>MYFFSVDPRNGASKSGDVCGSCCCESISARPGEVNGVMVSYAAWSAPLRGHGLTNKTTFEIDGVSVTPPKVSNAFGRTKVGVVFEGTLSDLFPNPEGEQVEYEISELNGPSNGVVELGANGAFTYTPGALFTGVDRFWFSINGNIGEYVISVDPTTSELPQPPFTTPVYVPAARRSVDPRTHVLKFVLGVSPAAIPGDVYRLTVRQVAIDCDGNEFVHISCYDISIGSCG[60x];>MNLDTLLPLQTIREHAKCDDNPRVTDDLLKLYREAAFEAAELYTGLSFTPEKTIVEPIRLKGRRGKIILSATPIAGRPVVFYGGGLGSPLELIPRPGSNVLFFPYGSPDRFQTWGDCHTCDVESQLMATYVTGRRCENSVPAGIIIGILKLIAWNINNPGDEVMSVRNTLNANAQGLIGGTNNGAVISGAQDEWFRYRRVLL[5x];>MVKLNCRPLCQAPTASRLVSPPCFICRGVAPSAPVTPG[25x];>[5x]MDCRNLCGAAAPSRLVQPGCFICRGVAVSIPPAAPGPATSVFDTPPSTFSLRPDGTIIAGTGIRGDHASVGTDGTIEMFIVPFIGDVTGSELTHPYAVELQDGEELAIAFGVTLKSGYGARITEYYDVSLFLENGGNSKELTLQPANTKSGYVWSDGHGYNITDSDGDLHTVQNVTRPVWFEMTEPGIVGVIMEARYKATGLVSSSISITVNVTYAD;>MANKESELNGLDDIHSDIEKLSAHVEKFSDGMDEKYKELTARFDGVKGDNDAIRKAVADATKEYAELSAKHQFFTEELAAMKARLDTPIMRSQAELDDHDRKTAIQLQRNMHEFRGGDPKEFVADESNLVDLKAYRSAVRKMLKVGIESKERVIASMTDVERKAFEASTIGPAFFTPQVLALEVDCNIECASLLDLYGQIEVSRSTFTYMKIADYGQLGEYTCDAKCDAEFGEPGNIRHLEGKTYDYRGVFCFNRKNLQEANYDFLSFMIGAAQRSHRINRNQALMIGKGVNEPKGWLTENCFPVFQTLPVDVNGTSTPAFLAQDWRRFVTSFPAEYGEARSVMHQNVFGYLAAMVDANGRFLFGDGDLTFTPDLVRERIRISNCLPDPTEGNTKGGTGQDAFAAGSFVAAQAAWKTAFYAVEKRPMFFEQYEGGSSAWCVKYQFGAEDGGFVGCCEHGRILQIG[30x];>MNFNVGVDFPSFIAWDGEESFPVKVDGFNQFGFTFKTIAALTAATTFNIFYHEPSDADPCVPGPAIRVPEVPFCDTVLLSEDGLAAVTLPETVTPDSFCAGTVPCMNGQWISIAPATGSETNAANVQITVTMKGATR[40x]

Caudovirales, the taxonomic order for the tailed double-stranded DNA bacteriophages, is characterized by the presence of a tail—a host cell attachment organelle that is connected to the genome-containing spherical or elongated capsid via a neck. We describe cryo-EM structures of the neck, the neck-capsid and neck-tail junctions, and capsid of the Agrobacterium phage Milano. The tail to capsid junction involves a symmetry mismatch that is bridged by the neck, and is therefore crucial for the assembly of tailed phage. The extensive network of disulfide bonds within and between neck, collar, capsid and tail provides an exceptional structural stability to Milano.

The 5-fold symmetrized map was used to build the model of the neck-capsid junction — the neck 1 and collar interacting with the 5-fold capsid vertex. Since this pentadecamer has both the C5 symmetry of the capsid and a C3 symmetry (present in the C6 symmetry of the tail), it is resolved in both the C3 and C5 symmetric reconstructions of the neck. The peripheral ring of neck 1 breaks the C12 symmetry of the core and connects the neck to the capsid. Our work characterizes how the β-sandwich domains of Milano neck 1 protomers (gp14) adopt different conformations to compensate for the head-to-neck symmetry mismatch and bridge them covalently. Five out of 12 gp14 β-sandwich domains (n, n + 2, n + 5, n + 7, n + 10, CCW direction looking from the capsid side) display pseudo-5-fold symmetry. These domains are covalently linked to the MCP (gp9) by two disulfide bonds, gp14Cys117– gp9Cys252 and gp14Cys120– gp9Cys440, which emanate from a head joining loop of the β-sandwich domains. The head joining loops of the remaining seven gp14 protomers are not resolved in our maps and thus likely to be disordered. Every third (n, n + 3, n + 6, n + 9, n + 12) collar subunit is attached to the neck 1 subunits (n, n + 2, n + 5, n + 7, n + 10, CCW direction looking from the capsid side) through the disulfide bond gp14Cys136—gp13Cys19, linking the collar to neck 1 by five disulfide bonds.> MPFLSSPSNSVSTYYEDHGDARSYPLVLIHPIGGNILIWDYEIQLLLKSGFRVIAYELRGHHRTNMGKTGAYTMQDLIDDLRRLLEHLNIGKCTIIGHSIGGIISSMYAAQHPG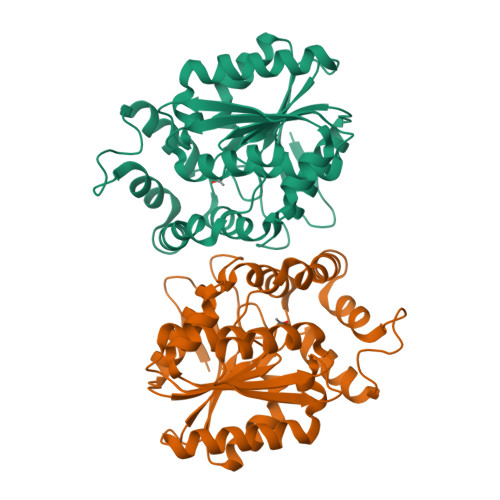KVDAIIMINGSPKKFQEKDLEKHFRTREVAITQGMKALAEHKLVSLDEARDLFADKRHADFFREVFTKTSVEGFVAATVALYTIPGNVVQGLRASGCKVFAIVGSDDDVFMRLIKETKEEIPEMELRVLQGSDHWVVIEKPKEMYDILMGFLAIVTKDVKPVG>[2x]MRCLALDIGGTKIASAIVTDGKIEQRQQIATPQADAANAMHDTLANILALYAGQFDYVAVASTGIINHGVLTALNPKNLGGLAEFPLKESIARHTDKPIGLLNDVQAAACAEYKDEDKN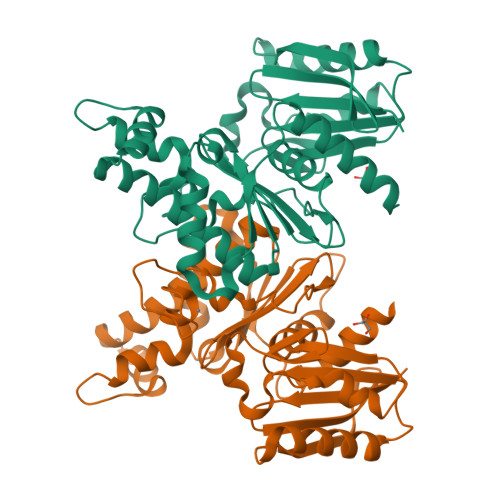AVQNFVFITVSTGVGGGIILERRLLTEPNGVAGHIGHTLADPNGPVCGCGRVGCVEAVAAGRAIEAVSSQWNPPCTPKQAFELFRKNDEKATALIQRSASAIANLIADLVIGLDVQKVVVGGSVGLAEGYLPLVKQYLNTMPHFYHCTVEQARHGQDAGLLGAAWWVADCLKQGVHLK> VKDTYTDRLDDWNGIIAGNQYYDSKNDQMAKLNQELEGKVADSLSSISSQADRIYLWEKFSNYKTSANLTATYRKLEEMAKQVTNPSSRYYQDETVVRTVRDSMEWMHKHVYNSEKSIVGNWWDYEIGTPRAINNTLSLMKEYFSDEEIKKYTDVIEKFVPDPEHFRKTTDNPFKALGGNLVDMGRVKVIAGLLRKDDQEISSTIRSIEQVFKLVDQGEGFYQDGSYIDHTNVAYTGAYGNVLIDGLSQLLPVIQKTKNPIDKDKMQTMYHWIDKSFAPLLVNGELMDMSRGRSISRANSEGHVAAVEVLRGIHRIADMSEGETKQRLQSLVKTIVQSDSYYDVFKNLKTYKDISLMQSLLSDAGVASVPRTSYLSAFNKMDKTAMYNAEKGFGFGLSLFSSRTLNYEHMNKENKRGWYTSDGMFYLYNGDLSHYSDGYWPTVNPYKMPGTTETDAKRADSDTGKVLPSAFVGTSKLDDANATATMDFTNWNQTLTAHKSWFMLKDKIAFLGSNIQNTSTDTAATTIDQRKLESSNPYKVYVNDKEASLTEQEKDYPETQSVFLESSDSKKNIGYFFFKKSSISMSKALQKGAWKDINEGQSDKEVENE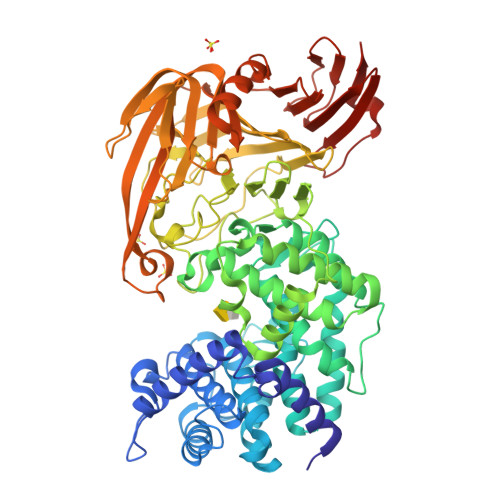FLTISQAHKQNGDSYGYMLIPNVDRATFNQMIKELESSLIENNETLQSVYDAKQGVWGIVKYDDSVSTISNQFQVLKRGVYTIRKEGDEYKIAYYNPETQESAPDQEVFKKLEQHHHHHH(2S,3S,4S,5R,6R)-2-(hydroxymethyl)-6-[[(2R,3S,4S,5R,6S)-6-[(3R,6S)-6-[(3S,8S,9R,10R,11S,13R,14S,17S)-3-[(2R,3R,4S,5S,6S)-6-(hydroxymethyl)-3,4,5-tris(oxidanyl)oxan-2-yl]oxy-4,4,9,13,14-pentamethyl-11-oxidanyl-2,3,7,8,10,11,12,15,16,17-decahydro-1H-cyclopenta[a]phenanthren-17-yl]-2-methyl-2-oxidanyl-heptan-3-yl]oxy-3,4,5-tris(oxidanyl)oxan-2-yl]methoxy]oxane-3,4,5-triol 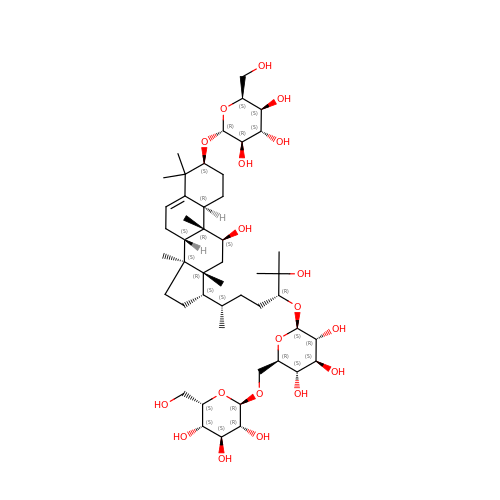| C48 H82 O19 | KYVIPFHNYCKOMQ-YDYRNPCOSA-N> MEHLYIVSYDIRNQRRWRRLFKTMHGFGCWLQLSVFQCRLDRIRIIKMEAAINEIVNHAEDHVLILDLGPAENV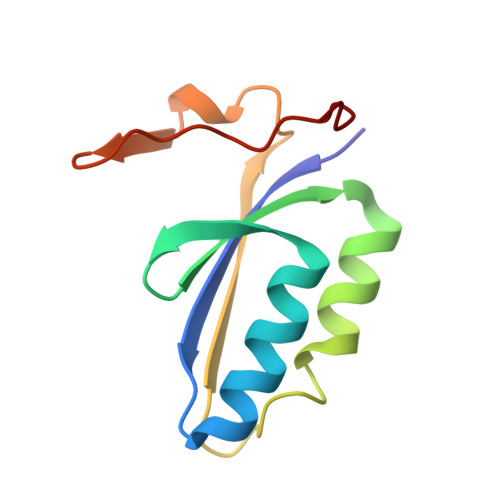KPKVSSIGKTFDPILRQAVIV> MALEEAPWPPPEGAFVGFVLSRKEPMWADLLALAAARGGRVHRAPEPYKALRDLKEARGLLAKDLSVLALREGLGLPPGDDPMLLAYLLDPSNTTPEGVARRYGGEWTEEAGERAALSERLFANLWGRLEGEERLLWLYREVERPLSAVLAHMEATGVRLDVAYLRALSLEVAEEIARLEAEVFRLAGHPFNLNSRDQLERVLFDELGLPAIGKTEKTGKRSTSAAVLEALREAHPIVEKILQYRELTKLKSTYIDPLPDLIHPRTGRLHTRFNQTATATGRLSSSDPNLQNIPVRTPLGQRIRRAFIAEEGWLLVALDYSQIELRVLAHLSGDENLIRVFQEGRDIHTETASWMFGVPREAVDPLMRRAAKTINFGVLYGMSAHRLSQELAIPYEEAQAFIERYFQSFPKVRAWIEKTLEEGRRRGYVETLFGRRRYVPDLEARVKSVREAAERMAFNMPVQGTAADLMKLAMVKLFPRLEEMGARMLLQVHDELVLEAPKERAEAVARLAKEVMEGVYP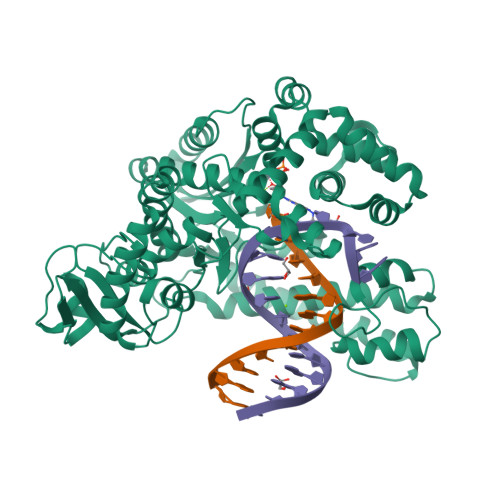LAVPLEVEVGIGEDWLSAKE>[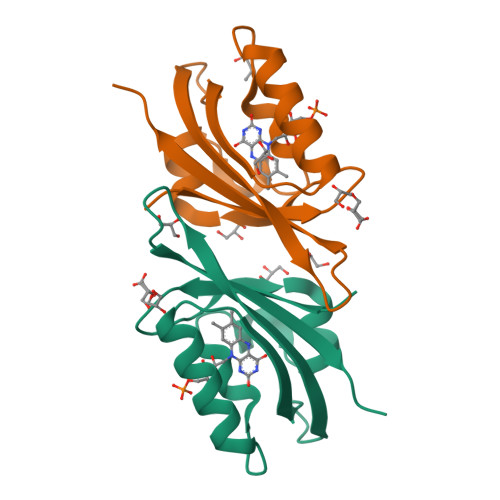2x]MASGMVVTDAGPDYPIIFANRAFSAITGYGPDEILGRNARFLQGPQTDWAVVARIREAIAAARPIHTRLLNYRKDGQPFWSQLAISPVRDETEQVVAFVGLQTDVTAHHHHHH> TGGVQTVTLIPGDGIGPEISAAVMKIFDAAKAPIQWEERNVTAIQGPGGKWMIPSEAKESMDKNKMGLKGPLKTPIAAGHPSMNLLLRKTFDLYANVRPCVSIEGYKTPYTDVNIVTIRENTEGEYSGIEHVIVDGVVASIKLITEGASKRIAEFAFEYARNNHRSNVTAVHKANIMRMSDGLFLQKCREVAESCKDIKFNEMYLDTVCLNMVQDPSQFDVLVMPNLYGDILSDLCAGLIGGLGVTPSGNIGANGVAIFESVHGTAPDIAGKDMANPTALLLSAVMMLRHMGLFDHAARIEAACFATIKDGKSLTKDLGGNAKCSDFTEEICRRVKDLD;> ASRSQAEDVRVEGSFPVTMLPGDGVGPELMHAVKEVFKAAAVPVEFQEHHLSEVQNMASEEKLEQVLSSMKENKVAIIGKIHTPMEYKGELASYDMRLRRKLDLFANVVHVKSLPGYMTRHNNLDLVIIREQTEGEYSSLEHESARGVIECLKIVTRAKSQRIAKFAFDYATKKGRGKVTAVHKANIMKLGDGLFLQCCEEVAELYPKIKFETMIIDNCCMQLVQNPYQFDVLVMPNLYGNIIDNLAAGLVGGAGVVPGESYSAEYAVFETGARHPFAQAVGRNIANPTAMLLSASNM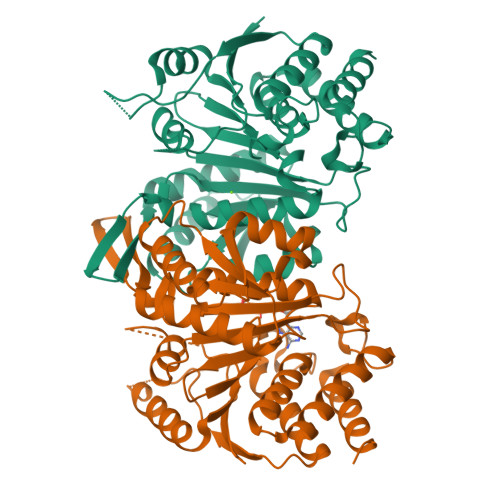LRHLNLEYHSSMIADAVKKVIKVGKVRTSDMGGYATCHDFTEEICRRVKDLDEN>[2x]MAHHHHHHMASLTVPAHVPSAAEDCEQL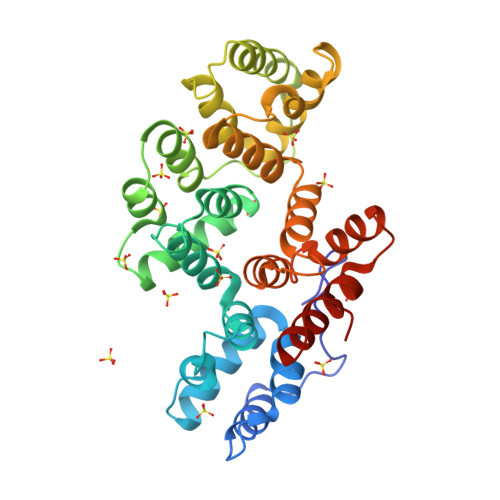RSAFKGWGTNEKLIISILAHRTAAQRKLIRQTYAETFGEDLLKELDRELTHDFEKLVLVWTLDPSERDAHLAKEATKRWTKSNFVLVELACTRSPKELVLAREAYHARYKKSLEEDVAYHTTGDHRKLLVPLVSSYRYGGEEVDLRLAKAESKILHEKISDKAYSDDEVIRILATRSKAQLNATLNHYKDEHGEDILKQLEDGDEFVALLRATIKGLVYPEHYFVEVLRDAINRRGTEEDHLTRVIATRAEVDLKIIADEYQKRDSIPLGRAIAKDTRGDYESMLLALLGQEED>[2x]TPDRHQFPGLANKTYFNFGGQGILPTVALEAITAM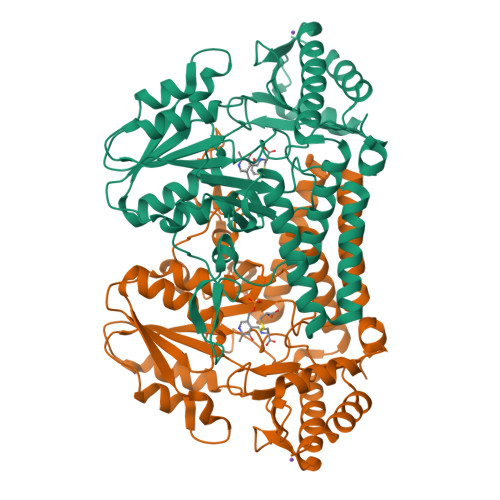YGYLQENGPFSIAANQHIQQLIAQLRQALAETFNVDPNTITITDNVTTGCDIVLWGLDWHQGDEILLTDCEHPGIIAIVQAIAARFGITYRFFPVAATLNQGDAAAVLANHLGPKTRLVILSHLLWNTGQVLPLAEIMAVCRRHQGNYPVRVLVDGAQSAGSLPLDFSRLEVDYYAFTGHAWFAGPAGVGGLYIHGDCLGEINPTYVGWRSITYGAKGEPTGWAEGGKRFEVATSAYPQYAGLLAALQLHQRQGTAEERYQAICQRSEFLWRGLNQLPHVHCLATSAPQAGLVSFTVDSPLGHRAIVQKLEEQRIYLRTIADPDCIRACCHYITDEEEINHLLARLADFGP> GSHMSQSNRELVVDFLSYKLSQKGYSWSQFSDVEENRTEAPEETESAVKQALREAGDEFELRYRRAFSDLTSQLHIT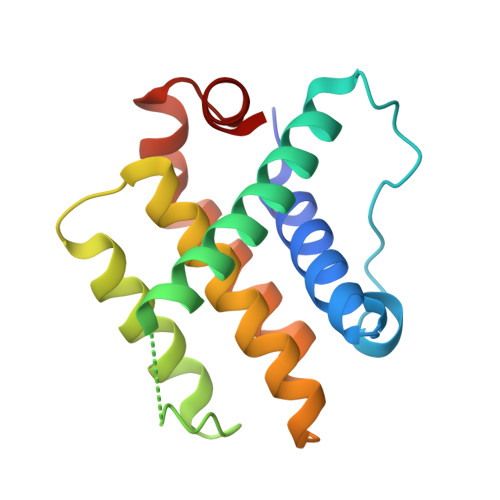PGTAYQSFEQVVNELFRDGVNWGRIVAFFSFGGALCVESVDKEMQVLVSRIASWMATYLNDHLEPWIQENGGWDTFVDLYG>[4x]GSHMADSSSSSFFPDFGLLLYLEELNKEELNTFKLFLKETMEPEHGLTPWNEVKKARREDLANLMKKYYPGEKAWSVSLKIFGKMNLKVLCERAKEEINWSAQLE

Here, crystal structures of human NLRP14 pyrin-domain variants are reported. Structurally, NLRPs share a conserved tripartite domain architecture consisting of an N-terminal pyrin domain, a central NACHT domain (with reference to its initial identification in NAIP, CIITA, Het-E and TP1) and a C-terminal leucine-rich repeat (LRR) domain. Pyrin domains belong to the death-domain superfamily, which includes the CARDs, the death-effector domains (DEDs) and the death domains (DDs) in addition to the PYDs. The death-domain fold consists of six antiparallel α-helices packed around a highly conserved hydrophobic core with Greek-key topology.

To this end, we crystallized the D86V mutant. Consequently, the clinical D86V mutation of NLRP14 PYD apparently does not affect its three-dimensional structure in comparison to the wild-type protein. We should note that despite a large variation of chemical space, all wild-type and D86V crystals belonged to the hexagonal space group P63 with four molecules per asymmetric unit, resembling a dimer of dimers. The charge-bridging system is similarly broken as in the wild-type protein, suggesting that this mutant could undergo the conformational switching necessary for dimerization. Indeed, the D86V mutant showed a very similar dimerization tendency to that observed for the wild-type protein. Remarkably, however, the D86V mutant revealed a higher tendency towards aggregation, as indicated by the pronounced void peak. While the engineered L84R mutant showed remarkable properties such as a drastically improved thermal stability that correlates with a strictly monomeric six-α-helix structure, the naturally occurring D86V mutant behaved very much like the wild-type protein despite its severe physiological implications. This suggested that the mechanistic basis for the physiological role of the D86V mutation should relate to its interaction with other relevant components rather than an intrinsic change within the pyrin-domain structure. By contrast, the negative charge is significantly reduced in this potential interface of the D86V mutant. Still, we emphasize that the proposed docking model merely serves to illustrate a possible mechanism for how the D86V mutation can severely affect the interaction of NLRP14 PYD with other binding partner molecules, even if ASC should turn out not to be the physiological binding partner of NLRP14 PYD.>[2x]AMGAPKPPQEPDMNNLPENPIPQHQAKFVLNTIKAVKRNREAVPFLHPVDTVKLNVPFYYNYIPRPMDLSTIERKINLKAYEDVSQVVDDFN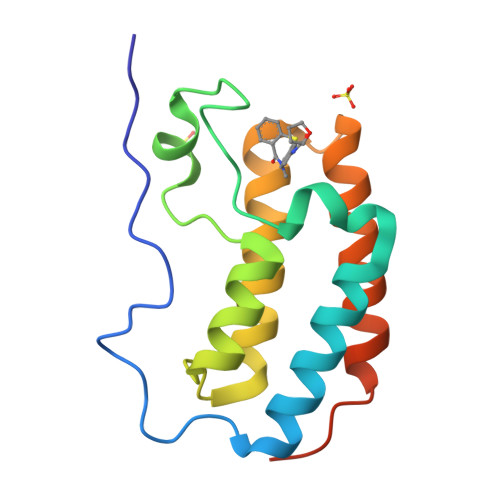LMVKNCKKFNGEAAGISKMATNIQAQFEKLMVKVPPKELPAGTNVA> GSGEFRIVPTTVALTMTLDKLDLPIVGKPTSYKTLPNRYKDVPEIGQPMEPNVEAVKKLKPTHVLSVSTIKDEMQPFYKQLNMKGYFYDFDSLKGMQKSITQLGDQFNRKAQAKELNDHLNSVKQKIENKAAKQKKHPKVLILMGVPGSYLVATDKSYIGDLVKIAGGENVIKVKDRQYISSNTENLLNINPDIILRLPH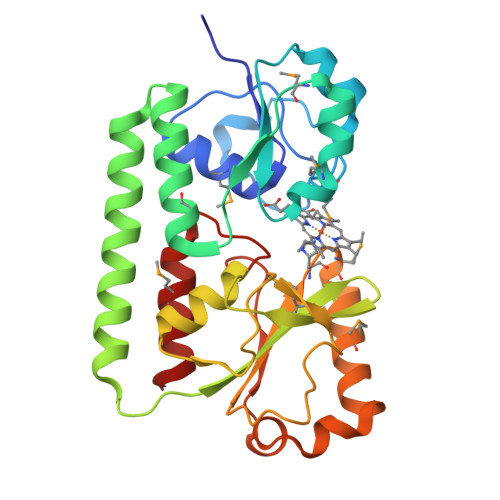GMPEEVKKMFQKEFKQNDIWKHFKAVKNNHVYDLEEVPFGITANVDADKAMTQLYDLFYK> GSAPLLLYANRRDLRLVDATNGKENATIVVGGLEDAAAVDFVFSHGLIYWSDVSEEAIKRTEFNKTESVQNVVVSGLLSPDGLACDWLGEKLYWTDSETNRIEVSNLDGSLRKVLFWQELDQPRAIALDPSSGFMYWTDWGEVPKIERAGMDGSSRFIIINSEIYWPNGLTLDYEEQKLYWADAKLNFIHKSNLDGTN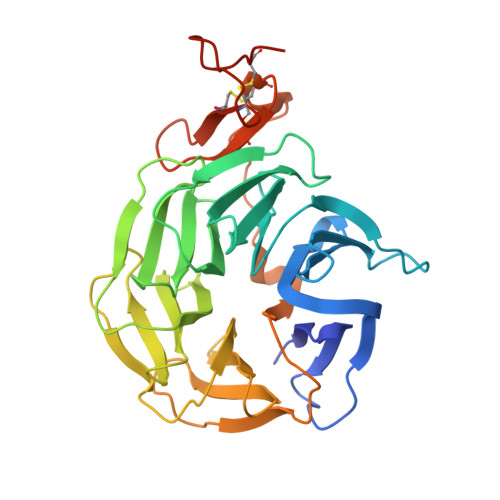RQAVVKGSLPHPFALTLFEDILYWTDWSTHSILACNKYTGEGLREIHSDIFSPMDIHAFSQQRQPNATNPCGIDNGGCSHLCLMSPVKPFYQCACPTGVKLLENGKTCKDGNSHHHHHH4-{4-[2-(4-fluorophenyl)-1,3-thiazol-4-yl]benzene-1-sulfonyl}morpholine | C19 H17 F N2 O3 S2 | 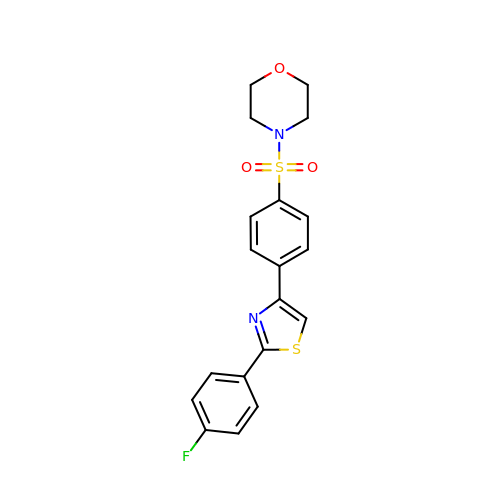JYTYZKKXJTUPJO-UHFFFAOYSA-N> EAEATDPNGYIVFCPCMGRFGNQVDQFLGVLAFAKALDRTLVLPNFIEFKHPETKMIPFEFLFQVGTVAKYTRVVTMQEFTKKIMPTVWPPEKRKAFCWTPRQAIYDKSAEPGCHSKEGNPFGPYWDQIDVSFVGDEYFGDIPGGFDLNQMGSRKKWLEKFPSEEYPVLAFSSAPAPFPSKGKVWSIQKYLRWSSRITEQAKKFISANLAKPFVAVHLRNDAD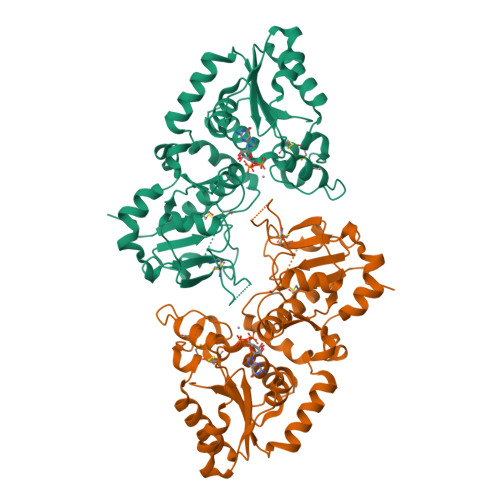WVRVCEHIDTTTNRPLFASEQCLGEGHHLGTLTKEICSPSKQQILEQIVEKVGSIGAKSVFVASDKDHMIDEINEALKPYEIEAHRQEPDDMYTSLAIMGRADLFVGNCVSTFSHIVKRERDHAGQSPRPSAFFGIRAV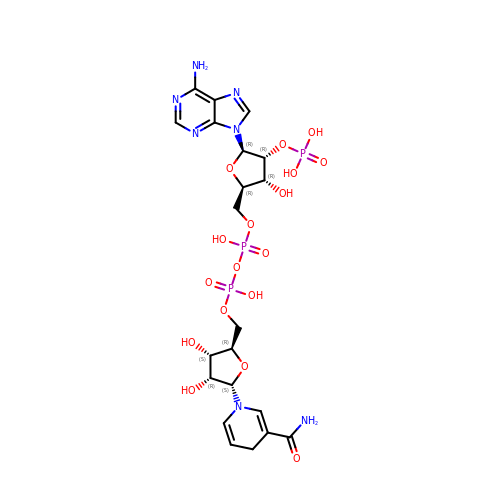alpha-NADPH | C21 H30 N7 O17 P3 | ACFIXJIJDZMPPO-OPDHFMQKSA-N>[2x]GTIYPRNPAMYSEEARLKSFQNWPDYAH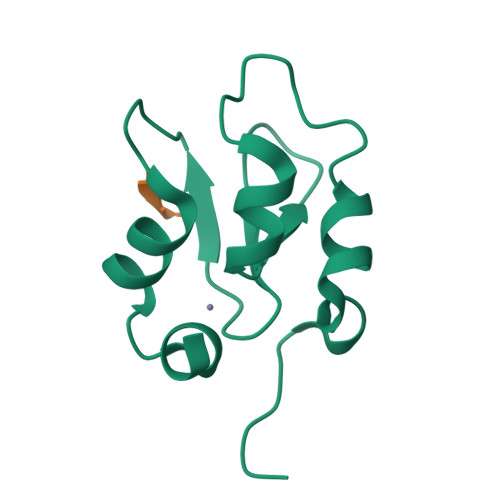LTPRELASAGLYYTGIGDQVQCFACGGKLKNWEPGDRAWSEHRRHFPNCFFVLGRNLN;> ATAA> MGDQRFGDLVFRQLAPNVWQHTSYLDMPGFGAVASNGLIVRDGGRVLVVDTAWTDDQTAQILNWIKQEINLPVALAVVTHAHQDKMGGMDALHAAGIATYANALS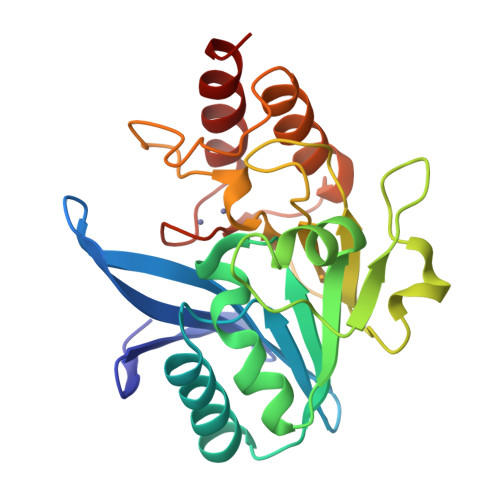NQLAPQEGLVAAQHSLTFAANGWVEPATAPNFGPLKVFYPGPGHTSDNITVGIDGTDIAFGGCLIKDSKAKSLGNLDDADTEHYAASARAFGAAFPKASMIVMSHSAPDSRAAITHTARMADKLR>MGSDKIHHHHHHMKSERILVVKTEDFLKEFGEFEGFMRVNFEDFLNFLDQYGFFRERDEAEYDETTKQVIPYVVIMDGDRVLITKRTTKQSEKRLHNLYSLGIGGHVREGDGATPREAFLKGLEREVNEEVDVSLRELEFLGLINSSTTEVSRVHLGALFLGRGKFFSVKEKDLFEWELIKLEELEKFSGVMEG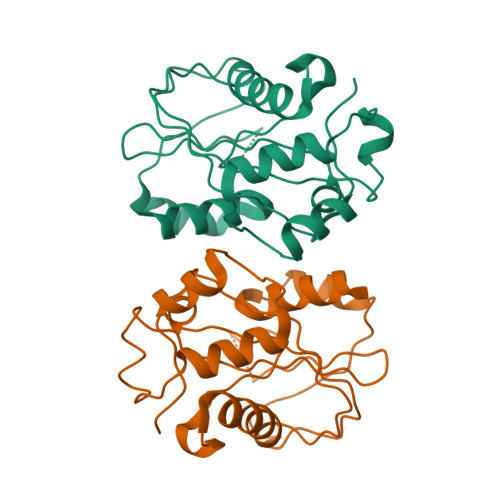WSKISAAVLLNLFLTQN[2x]>[4x]MVMALQTEQFNANILRNGEWVESRTGERISISAPASGVALGSIPALSQEEVNDAIQGAKDAQKIWKIRPIHERVDLLYAWADLLEERKEIIGELIMHEVAKPKKSAIGEVSRTADIIRHTADEALRLNGETLKGDQFKGGSSKKIALVEREPLGVVLAISP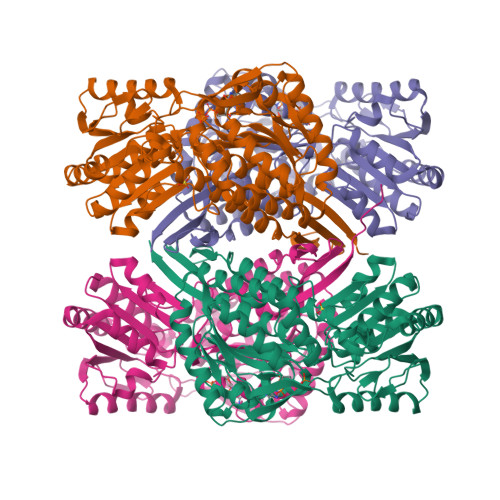FNYPVNLAAAKIAPALVTGNTVVFKPATQGSLSGIKMVEALADAGAPEGIIQVVTGRGSVIGDHLVEHPGIDMITFTGGTTTGERISEKAKMIPVVLELGGKDPAIVLDDADLKLTASQIVSGAFSYSGQRCTAIKRVFVQDSVADQLVANIKELVEQLTVGSPEDDADITPVIDEKSAAFIQGLIDDALENGATLLSGNKRQGNLLSPTLLDDVTPAMRVAWEEPFGPVLPIIRVKDANEAISLSNQSDYGLQASIFTKDTDRAINIGKHLEVGTVHINAKTERGPDHFPFLGVKKSGLGVQGIKPSLLSMTRERVTVLNLAENLYFQSHHHHHHWSHPQFEK>[2x]SSSSTASASAKKIIVKHVTVIGGGLMGAGIAQVAAATGHTVVLVDQTEDILAKSKKGIEESLRKVAKKKFA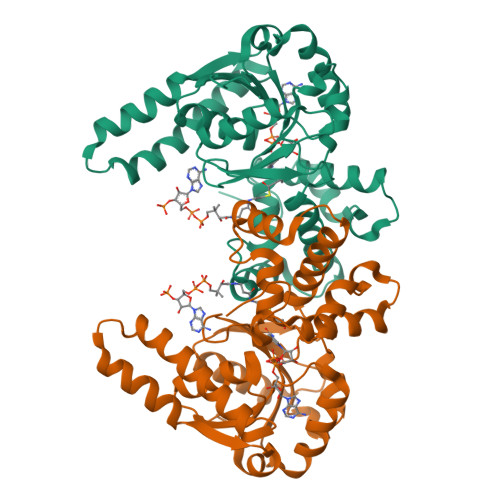ENPKAGDEFVEKTLSTIATSTDAASVVHSTDLVVEAIVENLKVKNELFKRLDKFAAEHTIFASNTSSLQITSIANATTRQDRFAGLHFFNPVPVMKLVQVIKTPMTSQKTFESLVDFSKALGKHPVSCKDTPGFIVNRLLVPYLMEAIRLYERGDASKEDIDTAMKLGAGYPMGPFELLDYVGLDTTKFIVDGWHEMDAENPLHQPSPSLNKLVAENKFGKKTGEGFYKYK(2E)-3-(3-chloro-5-{4-chloro-2-[2-(2,4-dioxo-3,4-dihydropyrimidin-1(2H)-yl)ethoxy]phenoxy}phenyl)prop-2-enenitrile 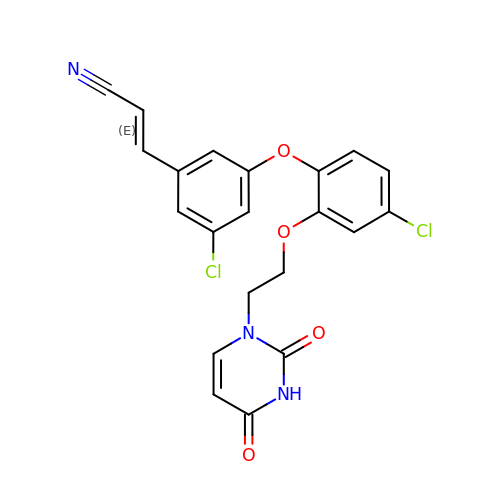| C21 H15 Cl2 N3 O4 | LXPGWIGXHHBGJC-OWOJBTEDSA-N>MAKKTSSKGKLPPGPTPLPFIGNYLQLNTEQMYNSLMKISERYGPVFTIHLGPRRVVVLCGHDAVREALVDQAEEFSGRGEQATFDWVFKGYGVVFSNGERAKQLRRFSIATLRDFGVGKRGIEERIQEEAGFLIDALRGTGGANIDPTFFLSRTVSNVISSIVFGDRFDYKDKEFLSLLRMMLGIFQFTSTSTGQLYEMFSSVMKHLPGPQQQAFQCLQGLEDFIAKKVEHNQRTLDPNSPRDFIDSFLIRMQEEEKNPNTEFYLK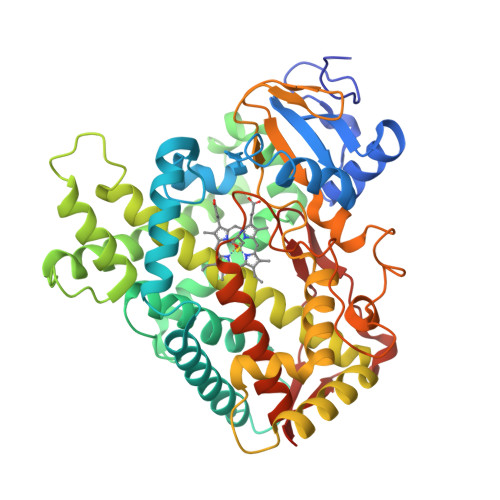NLVMTTLQLFIGGTETVSTTLRYGFLLLMKHPEVEAKVHEEIDRVIGKNRQPKFEDRAKMPYMEAVIHEIQRFGDVIPMSLARRVKKDTKFRDFFLPKGTEVYPMLGSVLRDPSFFSNPQDFNPQHFLNEKGQFKKSDAFVPFSIGKRNCFGEGLARMELFLFFTTVMQNFRLKSSQSPKDIDVSPKHVGFATIPRNYTMSFLPRHHHH[4x]>MRDVLEVLEFPRVRALLAERAKTPLGRELALALAPLPREEAEKRHELTGEALSYPYALPEAGTLREAYGRALAGARLSGPELLKAAKALEEAMALKEELLPLKNALSQVAEGIGDHTPFLERVRKALDEEGAVKDEASPRLAQIRRELRPLRQQILDRLYALMDRHREAFQDRFVTLRRERYCVPVRAGMAQKVPGILLDESESGATLFIEPFSVVKLNNRLQALRLKEEEEVNRILRDLSERLAKDEGVPKTLEALGLLDLVQAQAALARDLGLSRPAFGERYELYRAFHPLIPDAVRNSFALDEKNRILLISG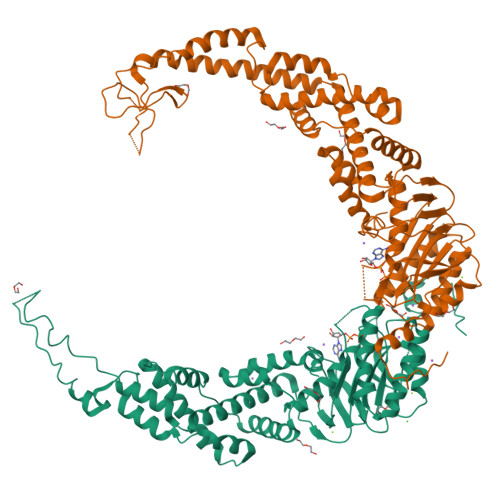PNMGGKTALLKTLGLAVLMAQSGLFVAAEKALLAWPDRVYADIGDEQSLQENLSTFAGHLRRLREMLEEATSHSLVLIDELGSGTDPEEGAALSQAILEALLERGVKGMVTTHLSPLKAFAQGREGIQNASMRFDLEALRPTYELVLGVPGRSYALAIARRLALPEEVLKRAE[2x]5-fluoro-N-(oxan-4-yl)pyridin-2-amine | C10 H13 F N2 O | 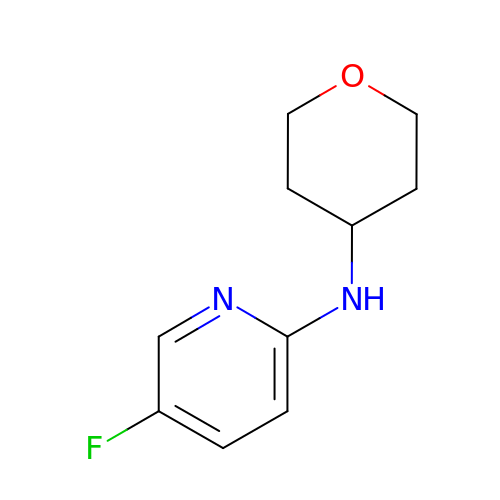DGYWCGILBGNERL-UHFFFAOYSA-N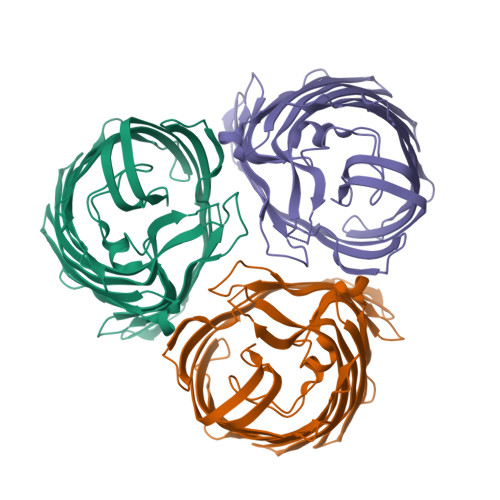> DAGTVDFYGQLRTELKFLEDKDPTIGSGSSRAGVDANYTVNDSLALQGKVEFALKDSGDMYVRNHILGVKTNFGKFSFGKQWTTSDDVYGADYSYFFGGTGLRYGTLSDALHDSQVKYVYEADSFWVKAGYGFPEDNAKQELAELYVGATFGDLAVHAGGGQNRDKAFKVGSNTVGTTTTDIKADVTNSYFEVTGEYTIGDALIGVTYYNAELDVENNPLVIDEDAISVAGTYKVADKTKLYAGYEYVMQEANTGADEDGTLVYLGVEYKFASWARVYAEYGYGDGTTLGYTNKGSDAEVKATKVDSANNFGIGARYYW>[2x]KEFTLDFSTAKTYVDSLNVIRSAIGTPLQTISSGGTSLLMIDSGTGDNLFAVDVRGIDPEEGRFNNLRLIVERNNLYVTGFVNRTNNVFYRFADFSHVTFPGTTAVTLSGDSSYTTLQRVAGISRT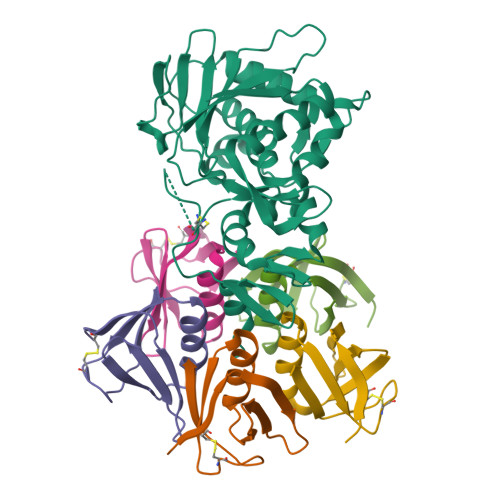GMQINRHSLTTSYLDLMSHSGTSLTQSVARAMLRFVTVTAEALRFRQIQRGFRTTLDDLSGRSYVMTAEDVDLTLNWGRLSSVLPDYHGQDSVRVGRISFGSINAILGSVALILNCHHHASRVARMASDEFPSMCPADGRVRGITHNKILWDSSTLGAILMRRTISS;>[10x]TPDCVTGKVEYTKYNDDDTFTVKVGDKELFTNRWNLQSLLLSAQITGMTVTIKTNACHNGGGFSEVIFR>MQNYNAKSIEVLTGLDPVKKRPGMYTNIENPNHLIQEIIDNSVDEVLAGFASKINITLYEDNSIEVADDGRGMPVDIHPEHKMSGIELIMTKLH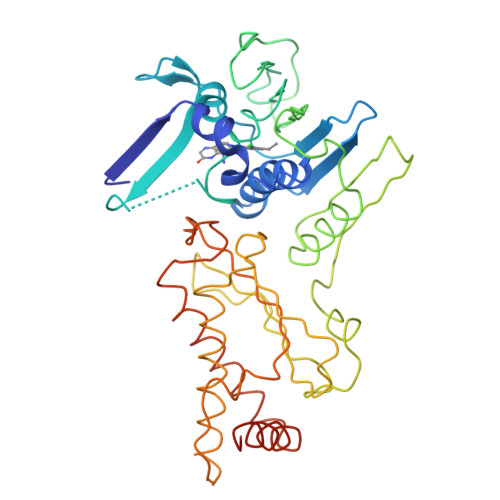SGGKFSNKNYTHSGGLHGVGVSVVNALSTRLEAEIKRDGNVYHIVFEDGFKTKDLEIIDNVGKKNTGTKIRFWPNKKYFDDIKVNFKALKNLLEAKAILCKALTIKYSNEIKKEKLTWHFETGLKGYLDHKLEAETLPAEPFIIDNFSNGDSYLDAVFCWCEDPSESIKNSYVNLIPTPQDGTHVTGLKNGIYDAIKAYIEKNSLSVKNIKITANDSFAQLNYVISVKITNPQFAGQTKEKLSNKDVTNFVATAVKDLLTIWLNQNPDEARQIVENISKVAQKRINADLEHHHHHH[2x]> MVGGYKVSNLTVEAFEGIGSVNPMLFYQYKVTGKGKYDNVYKIIKSARYKMHSKNRFKPVFIKDDKLYTLEKLPDIEDLDFANINFVKSEVLSIEDNMSIYGEVVEYYINLKLKKVKVLGKYPKYRINYSKEILSNTLLTRELKDEFKKSNKGFNLKRKFRISPVVNKMGKVILYLSCSADFSTNKNIYEMLKEGLEVEGLAVKSEWSNISGNLVIESVLETKISEPTSLGQSLIDYYKNNNQGYRVKDFTDEDLNANIVNVRGNKKIYMYIPHALKPIITREYLAKNDPEFSKEIEQLIKMNMNYRYETLKSFVNDIGVIEELNNLSFKNKYYEDVKLLGYSSGKIDEPVLMGAKGIIKNKMQIFSNGFYKLPEGKVRFGVLYPKEFDGVSRKAIRAIYDFSKEGKYHGESNKYIAEHLINVEFNPKECIFEGYELGDITEYKKAALKLNNYNNVDFVIAIVPNMSDEEIE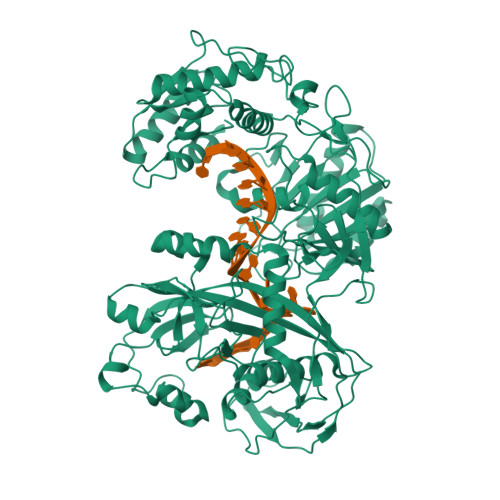NSYNPFKKIWAELNLPSQMISVKTAEIFANSRDNTALYYLHNIVLGILGKIGGIPWVVKDMKGDVDCFVGLDVGTREKGIHYPACSVVFDKYGKLINYYKPNIPQNGEKINTEILQEIFDKVLISYEEENGAYPKNIVIHRDGFSREDLDWYENYFGKKNIKFNIIEVKKSTPLKIASINEGNITNPEKGSYILRGNKAYMVTTDIKENLGSPKPLKIEKSYGDIDMLTALSQIYALTQIHVGATKSLRLPITTGYADKICKAIEFIPQGRVDNRLFFL> GSPGISGGGGGILDSMDVVSLDKPFMYFEEIDNELDYEPESANEVAKKLPYQGQLKLLLGELFFLSKLQRHGILDGATVVYIGSAPGTHIRYLRDHFYNLGVIIKWMLIDGRHHDPILNGLRDVTLVTRFVDEEYLRSIKKQLHPSKIIL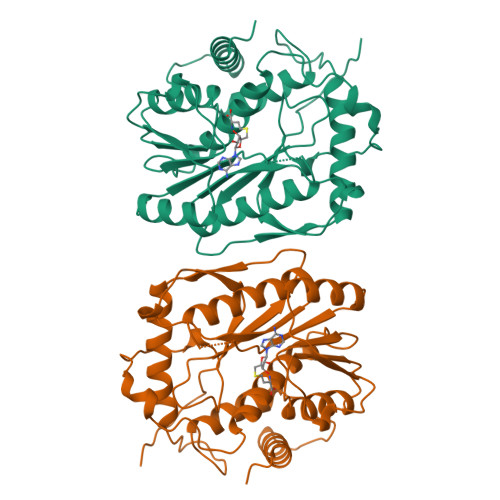ISDVRSKRGGNEPSTADLLSNYALQNVMISILNPVASSLKWRCPFPDQWIKDFYIPHGNKMLQPFAPSYSAEMRLLSIYTGENMRLTRVTKSDAVNYEKKMYYLNKIVRNKVVVNFDYPNQEYDYFHMYFMLRTVYCNKTFPTTKAKVLFLQQSIFRFLNIPTTSTEKVSHEPIQRKISSKNSMSKNRNSKRSVRSNK>[6x]MSGPAHLPYGGIPTFARAPLVQPDGDWQADVAALGVPFDIALGFRPGARFAPRALREASLRSVPPFTGLDGKTRLQGVTFADAGDVILPSLEPQLAHDRITEAARQVRGRCRVPVFLGGDHSVSYPLLRAFADVPDLHVVQLDAHLDFTDTRNDTKWSNSSPFRRACEALPNLVHITTVGLRGLRFDPEAVA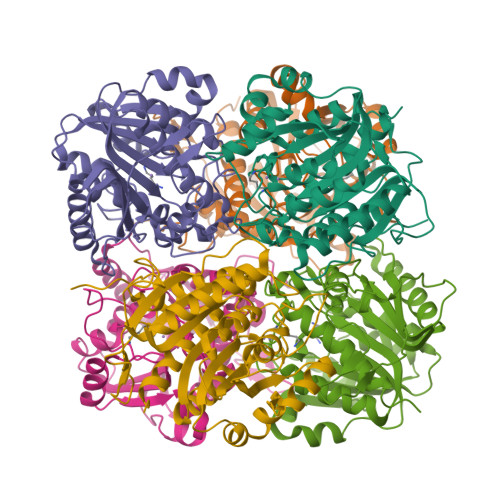AARARGHTIIPMDDVTADLAGVLAQLPRGQNVYFSVDVDGFDPAVIPGTSSPEPDGLTYAQGMKILAAAAANNTVVGLDLVELAPNLDPTGRSELLMARLVMETLCEVFDHVL> MFCEKAMELIRELHRAPEGQLPAFNEDGLRQVLEEMKALYEQNQSDVNEAKSGGRSDLIPTIKFRHCSLLRNRRCTVAYLYDRLLRIRALRWEYGSVL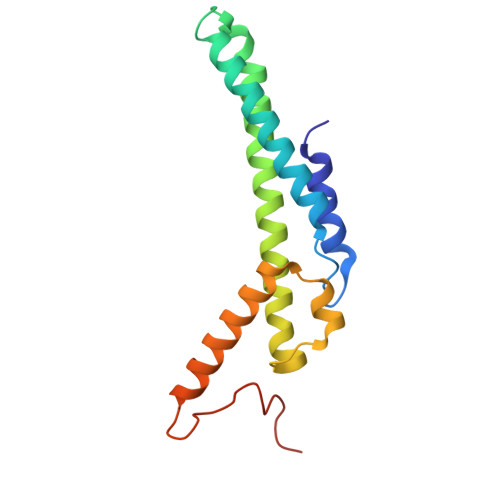PNALRFHMAAEEMEWFNNYKRSLATYMRSLGGDEGLDITQDMKPPKSLYIE>MHHHHHHVSHDDLMLALALADRADELTRVRFGALDLRIDTKPDLTPVTDADRAVESDVRQTLGRDRPGDGVLGEEFGGSTTFTGRQWIVDPIDGTKNFVRGVPVWASLIALLEDGVPSVGVVSAPALQRRWWAARGRGAFASVDGARPHRLSVSSVAELHSASLSFSSLSGWARPGLRERFIGLTDTVWRVRAYGDFLSYCLVAEGAVDIAAEPQVSVWDLAALDIVVREAGGRLTSLDGVAGPHGGSAVATNGLLHDEVLT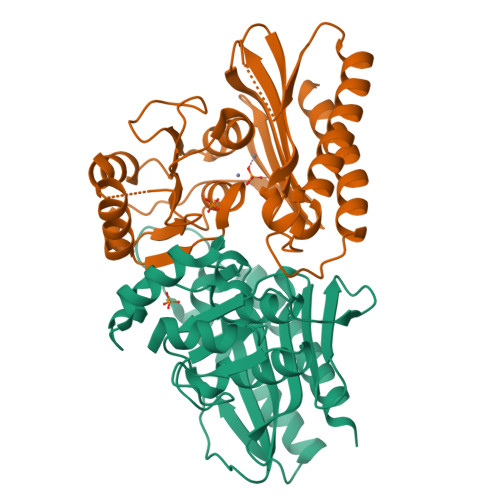RLNAG[4x]>GMSFDINWSTLESDNRLNDLIRKHLNSYLQNTQLPSYVSNLRVLDFDLGKVGPAITLKEITDPLDEFYDSIREEGGSGGSPNDIQFLLEVEYKGDLLVTIGADLVLNYPVEKFMTLPVKLSISDIGLHSLCIVACLSKQLFLSFLCDVSDPALDDNQTVLDPKGPILAATKPLERISIVRSMKIETEIGEQYQGQGSVLRSVGELEQFLFTI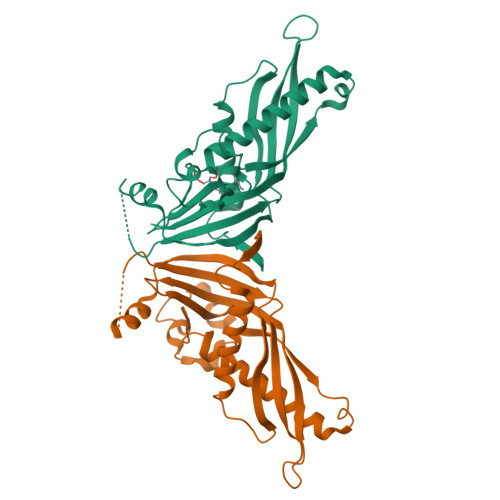FKDFLRKELAWPSWINLDFNDGDE[6x]>MAGDTTITIVGNLTADPELRFTSSGAAVVNFTVASTPRIYDRQSGEWKDGEALFLR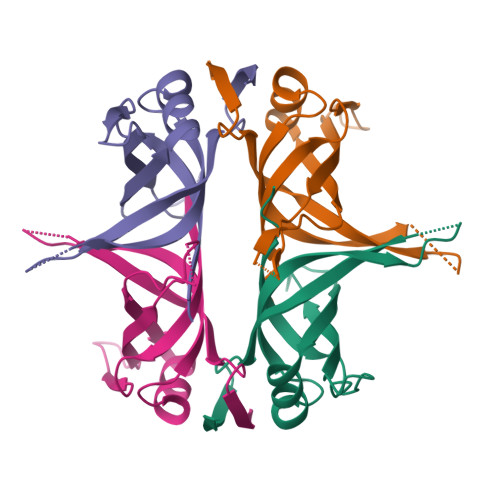CNIWREAAENVAESLTRGARVIVTGRLKQRSFETREGEKRTVVEVEVDEIGPSLRYATAKVNKASRSGGGGGGFGSGSRQAPAQMSGGVGDDPWGSAPTSGSFGVGDEEPPF[4x]>[2x]GPLGSMGKKSRVKTQKSGTGATATVSPKEILNLTSELLQKCSSPAPGPGKEWEEYVQIRTLVEKIRKKQKGLSVTFDGKREDYFPDLMKWASENGASVEGFEMVNFKEEGFGLRATRDIKAEELFLWVPRKLLMTVESAKNSVLGPLYSQDRILQAMGNIALAFHLLCERASPNSFWQPYIQTLPSEYDTPLYFEEDEVRYLQSTQAIHDVFSQYKNTARQYAYFYKVIQTHPHANKLPLKDSFTYEDYRWAVSS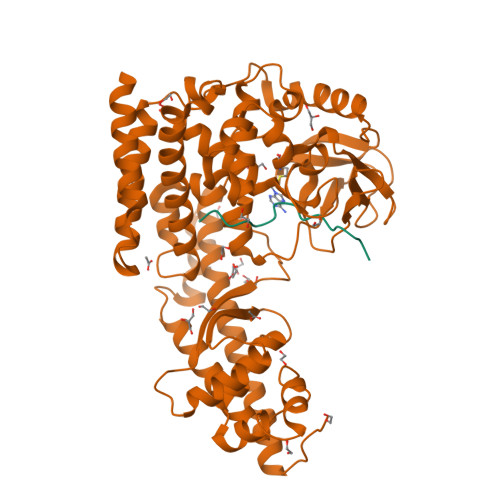VMTRQAQIPTEDGSRVTLALIPLWDMCNHTNGLITTGYNLEDDRCECVALQDFRAGEQIYIFYGTRSNAEFVIHSGFFFDNNSHDRVKIKLGVSKSDRLYAMKAEVLARAGIPTSSVFALHFTEPPISAQLLAFLRVFCMTEEELKEHLLGDSAIDRIFTLGNSEFPVSWDNEVKLWTFLEDRASLLLKTYKTTIEEDKSVLKNHDLSVRAKMAIKLRLGEKEILEKAVKSAAVNREYYRQQMEEKAPLPKYEESNLGLLESSVGDSRLPLVLRNLEEEAGVQDALNIREAISKAKATENGLVNGENSIPNGTRSENESLNQESKRAVEDAKGSSSDSTAGVKE;>[2x]TLKYPIEHGIVTNWD N-methyl-1-(4-phenoxyphenyl)methanamine 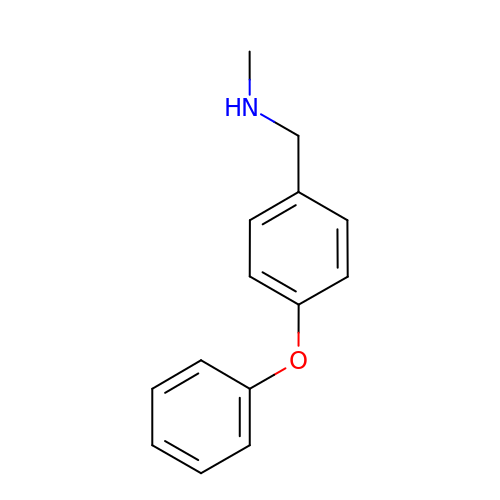| C14 H15 N O | YWBKPTGYRUSBFV-UHFFFAOYSA-N>[3x]MGKTYYMDPEGSDSNPGTSDKPFATLVKVQEVVVAGDVVYINPGTYVVPANQVPMTTTNSGLYHCVFHMNKSGEAGKPISYLANPNKQGRPIFDLSQVKPKDQRITVFYVTGSNLYLKGFDVIGTQVTITGHTQSECFRIVKGANNNKFEDLRTHDGMAIGFYLLGGSNNHILNCDAYNNYDSVSEGGKGGNVDGFGGHINSSSVGE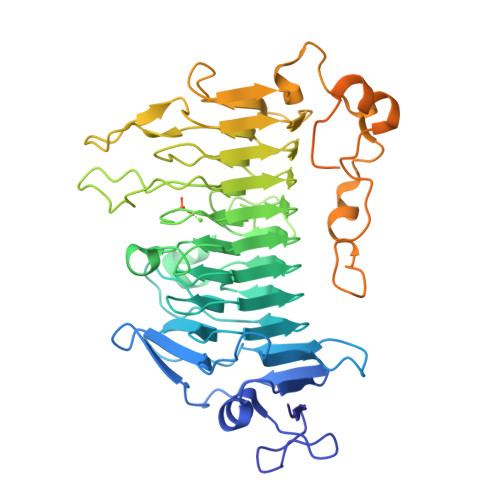GKGTGNVFEGCRAWYNSDDGFDLINCFEAVKIINCWSFLNGYKPGTKEVAGDGTGFKAGGYGMAADKLPAIPSVIPQHEVRNSLAYYNRLRGFYANHHLGGIIFESNTAVNSGENYNMTNRESPLALPPTDVNGYDHMVKNNLSLVTRSGSKHIVMVNRAKSEVSNNSFDGSEEVIETDFISLEEAELMRDRKPNGDLPDVNFGKLTTDAELRFWGMGCFATGEPTDLDFGWLKKPTIVVVGSKASVVGPEAASFTKMYVIVDGEETTEFDKNSIDLSDFSGVLEVKAVIEDANGNITKSIALKFKRLEHHHHHH>FKTIKSDEIFAAAQKLMPGGVSSPVRAFKSVGGQPIVFDRVKDAYAWDVDGNRYIDYVGTWGPAICGHAHPEVIEALKVAMEKGTSFGAPCALENVLAEMVNDAVPSIEMVRFVNSGTEACMAVLRLMRAYTGRDKIIKFEGCYHGHADMFLVKAGSGVATLGLPSSPGVPKKTTANTLTTPYNDLEAVKALFAENPGEIAGVILEPIVGNSGFIVPDAGFLEGLREITLEHDALLVFDEVITGFRIAYGGVQEKFGVTPDLTTLGKIIGGGLPVGAYGGKREIMQLVAPAGPMYQAGTLSGNPLAMTAGIKTLELLRQPGTYEYLDQITKRLSDGLLAIAQETGHAACGGQVSGMFGFFFTEGPVHNYEDAKKSDLQKFSRFHRGML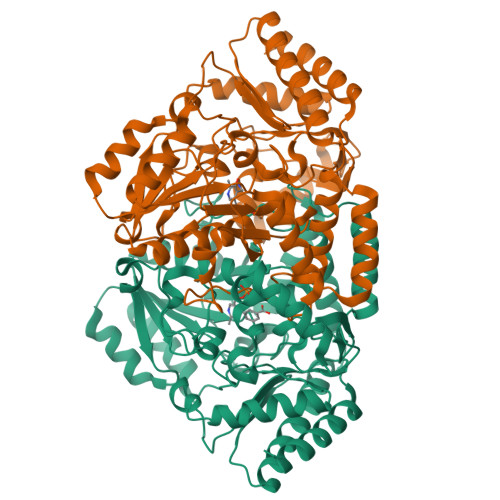EQGIYLAPSQFEAGFTSLAHTEEDIDATLAAARTVMSAL[2x]>MAKITFPKDFIWGSATAAYQIEGAYNEDGKGESIWDRFSHTPGNIADGHTGDVACDHYHRYEEDIKIMKEIGIKSYRFSISWPRIFPEGTGKLNQKGLDFYKRLTNLLLENGIMPAITLYHWDLPQKLQDKGGWKNRDTTDYFTEYSEVIFKNLGDIVPIWFTHNEPGVVSLLGHFLGIHAPGIKDLRTSLEVSHNLLLSHGKAVKLFREMNIDAQIGIALNLSYHYPASEKAEDIEAAELSFSLAGRWYLDPVLKGRYPENALKLYKKKGIELSFPEDDLKLISQPIDFIAFNNYSSEFIKYDPSSESGFSPANSILEKFEKTDMGWIIYPEGLYDLLMLLDRDYGKPNIVISENGAAFKDEIGSNGKIEDTKRIQYLKDYLTQAHRAIQDGVNLKAYYLWSLLDNFE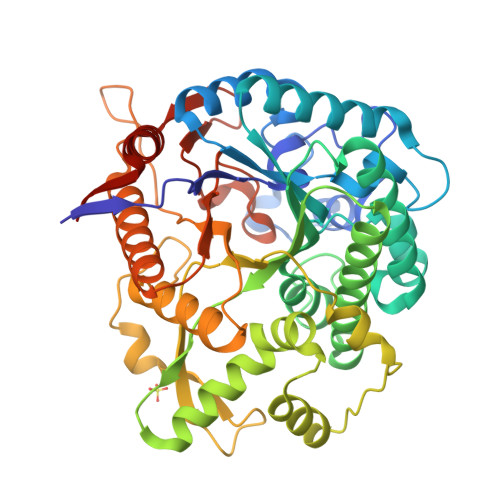WAYGYNKRFGIVHVNFDTLERKIKDSGYWYKEVIKNNGFLEHHHHHH[2x]~{N}-[(3~{R})-1,1-bis(oxidanylidene)thian-3-yl]-2-methyl-pyridin-3-amine | C11 H16 N2 O2 S 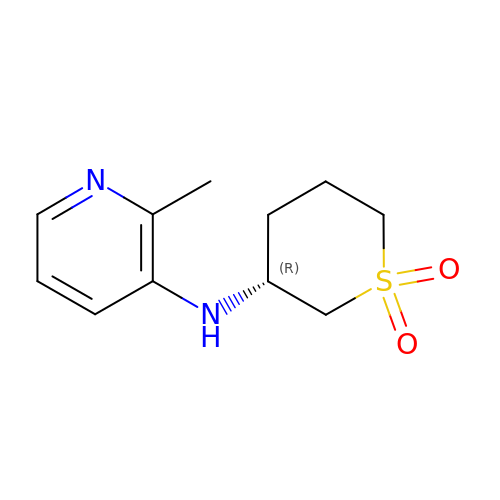| UTGFIRRMSACIPX-SNVBAGLBSA-N>MKKIEAIVRAEKFPEVKAALEERGFYGMTVTDVKGRGQQGGMQIQFRGRTMEVTLLPKVKLEIVVKDDAVEEVIGL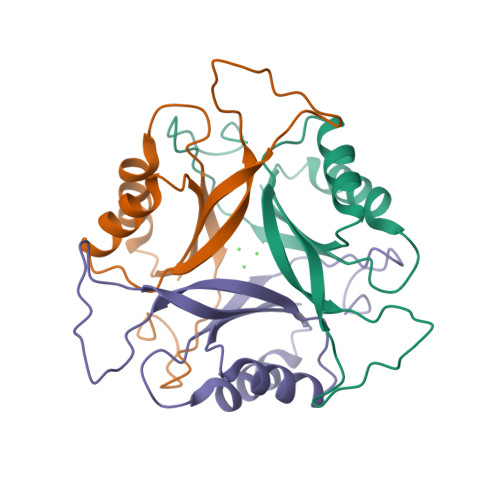IVNSAFTGSPGDGKIFIIPVEDVVRIRTGERGDDSLEHHHHHH[4x]>[4x]MIITVTLN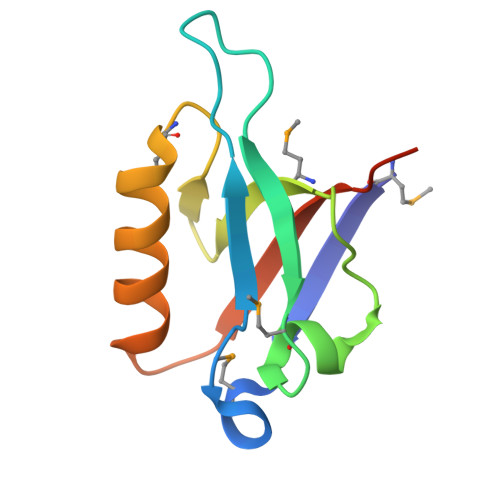MEKYNFLGISIVGQSNERGDGGIYIGSIMKGGAVAADGRIEPGDMLLQVNDINFENMSNDDAVRVLRDIVHKPGPIVLTVAKLEHHHHHH>ADPGEWPTHTVCKEENLEIYYKSCDPQQDFAFSIDRCSDVTTHTFDIRAAMVL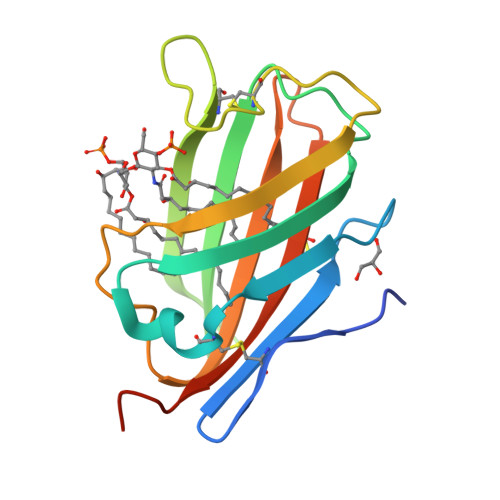RQSIKELYAKVDLIINGKTVLSYSETLCGPGLSKLIFCGKKKGEHLYYEGPITLGIKEIPQRDYTITARLTNEDRATVACADFTVKNYLDYSASLVPR[2x]FKBP8 consists of an N-terminal glutamate rich region and a PPIase domain that is connected by a loop to a tetratricopeptide domain (TPR). FKBP8 belongs to the FK506 family of binding proteins, but unlike many members of this family it lacks a constitutive PPIase activity, which instead relies on regulatory control. Activated FKBP8 has been shown to bind Bcl-2 and block its interaction with the pro-apoptotic protein, Bad, an activity which is inhibited by the molecular chaperone Hsp90. Here we have determined the structure of FKBP92-380, and shown that this TPR domain is specific for Hsp90 binding over Hsp70.

Crystals of FKBP92-380 in complex with yHsp90 DTEMEEVD peptide were obtained by mixing FKBP92-380 with yHsp90546-709 in a 1:1 molar ratio at 18 mg ml-1 and crystalizing by using the sitting drop vapour diffusion technique. The bound peptides found were DTEMEEVD, ATEMEEVD (where the side chain of the first aspartate residue was modeled as an alanine), EMEEVD and EMEE. Superimposition of FKBP92-380 with FKBP52 shows that the TPR domains are essentially the same consisting of three pairs of anti-parallel helices and a C-terminal α-7 helix. In contrast, a comparison with the MEEVD binding TPR domain of CHIP shows that the conformation of the Hsp90 peptide in both FKBP92-380 and CHIP is almost identical, and therefore similar to those also seen in AIP and Tah1. Because these structures share a common peptide polarity, and the hydrophobic methionine and the valine residues of the DTEMEEVD peptide are buried, as expected, in hydrophobic pockets, it is highly likely that this conformation represents the physiologically bound state for Hsp90 peptide. The structure of the FKBP92-380-Hsp90 peptide shows that the C-terminal carboxylate group and the C-terminal aspartate side-chain of the Hsp90 peptide are involved in a series of hydrogen bonds that is reminiscent of the carboxylate clamp seen in the MEEVD-HOP complex. The C-terminal carboxylic acid makes direct hydrogen bonds to the amine nitrogen of Asn 229 and Asn 277 and a salt bridge interaction to one of the amine nitrogen atoms of Arg 225, as well as water mediated interactions to the amine group of Lys 273. The aspartate group of the peptide makes a salt bridge interaction with the amine group of Lys 307 and a series of water mediated interactions with the amide groups of Asn 305, Asn 276 and Arg 311. Finally, the methionine side chain is bound in a hydrophobic pocket lined by Ile 306, Lys 307, Phe 310, Thr 341, Ile 342 and Asn 339.

>[4x]DTEMEEVD;>EEWLDILGNGLLRKKTLVPGPPGSSRPVKGQVVTVHLQTSLENGTRVQEEPELVFTLGDCDVIQALDLSVPLMDVGETAMVTADSKYCYGPQGRSPYIPPHAALCLEVTLKTAVDGPDLEMLTGQERVALANRKRECGNAHYQRADFVLAANSYDLAIKAITSSAKVDMTFEEEAQLLQLKVKCLNNLAASQLKLDHYRAALRSCSLVLEHQPDNIKALFRKGKVLAQQGEYSEAIPILRAALKLEPSNKTIHAELSKLVKKHAAQRSTETALYRKMLGNPSRLPAKCPG[4x]> TRKMWSVQESEWLKQGVVRYGVGHWERIRSAFPFAGRT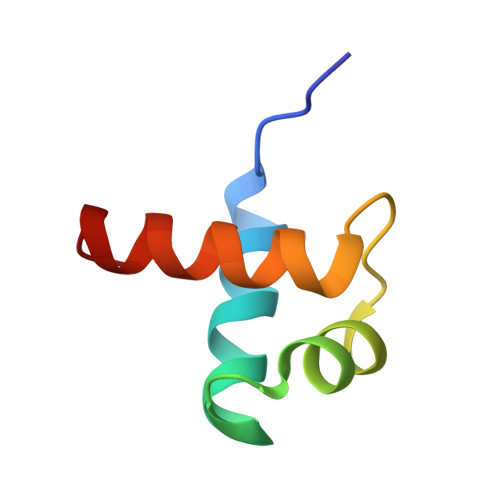AVNLKDRWRTMVKLKM Formation of active HIV-1 reverse transcriptase (RT) proceeds via a structural maturation process that involves subdomain rearrangements and formation of an asymmetric p66/p66′ homodimer. The viral RNA codes for a p66 protein that forms an asymmetric homodimer in which the RNase H domain in one subunit becomes destabilized, leading to subsequent unfolding and proteolysis in order to form the active p66/p51 heterodimer. We utilized the isolated polymerase domain, p51, rather than p66, since the initial subdomain rearrangements are largely limited to this domain. Two different fingers/palm/connection (FPC) subdomain constructs containing the same interfaces that are present in the monomers and in the p51 subunit of the RT heterodimer were investigated using both NMR spectroscopy and X-ray crystallography.

However, picrate, which gave a strong STD signal, was also found to promote crystallization. STD studies performed using the FPC construct identified picrate as a high-affinity ligand, and X-ray crystallography revealed a trio of picrate molecules bound to the fingers subdomain surface involved in dimer interface formation. The FPC–picrate complex contains a cluster of three picrate molecules located in a surface depression of the fingers subdomain between the β2–β3 and β7–β8 loops. The three negative charges are neutralized by residues Lys20, Lys22, and Arg143, with the latter forming a stacking interaction with picrate 1. The β7–β8 loop, which has been shown to play an important role in forming the interface with p66, follows a different trajectory in the presence of the picrate ligands. The well-defined picrate cluster was observed in two different crystal structures and defines a specific arrangement of the component picrate molecules. The picrate cluster also forms a lattice contact at which two FPC molecules interact, with the PIC3 molecule common to both clusters. Overlay of the FPC–picrate complex with the p51 subunit of RT indicates direct steric conflict with p66 residues Trp88 and Glu89 on the p66 αB-β5 loop. Additionally, the picrate 2 position conflicts with p51 residue Asn138. Thus, both direct steric competition with p66 and alteration of the positions of the β2–β3 and particularly the β7–β8 loop in p51 will interfere with dimerization.

> SDHHHHHHGPISPIETVPVKLKPGMDGPKVKQWPLTEEKIKALVEICTEMEKEGKISKIGPENPYNTPVFAIKKKDSTKWRKLVDFRELNKRTQDFWEVQLGIPHPAGLKKKKSVTVLDVGDAYFSVPLDEDFRKYTAFTIPSINNETPGIRYQYNVLPQGWKGSPAIFQSSMTKILEPFKKQNPDIVIYQYMDDLYVGSDLEIGQHRTKISELRQHLLRWGLTTPDGYELHPDKWTGSGSGGYDPSKDLIAEIQKQGQGQWTYQIYQEPSKNLKTGKYARMRGAHTNDVKQLTEAVQKITTESIVIWGKTPKFKLPIQKETWETWWTEYWQATWIPEWEFVN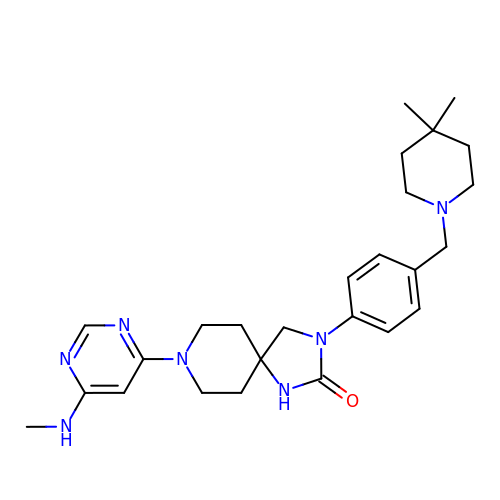3-[4-[(4,4-dimethylpiperidin-1-yl)methyl]phenyl]-8-[6-(methylamino)pyrimidin-4-yl]-1,3,8-triazaspiro[4.5]decan-2-one | C26 H37 N7 O | JSLLBTAATPZHSC-UHFFFAOYSA-N>DLVNLLRCQEGPRNCRELLSQGATLSGWYHLCLPEGRALPVFCDMDTEGGGWLVFQRRQDGSVDFFRSWSSYRAGFGNQESEFWLGNENLHQLTLQGNWELRVELEDFNGNRTFAHYATFRLLGEVDHYQLALGKFSEGTAGDSLSLHSGRPFTTYDADHDSSNSNCAVIVHGAWWYASCYRSNLNGRYAVSEAAAHKYGIDWASGRGVG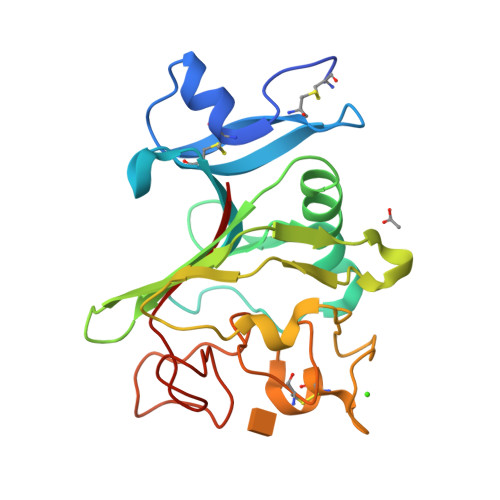HPYRRVRMMLR[3x]> MTARIALASLFVVAAVLAQPWQTTTQRWVLGVSIAAVIVLLAWWKGMFLTTRIGRALAMVRRNRAEDTVETDAHRATVVLRVDPAAPAQLPVVVGYLDRYGITCDKVRITHRDAGGTRRSWISL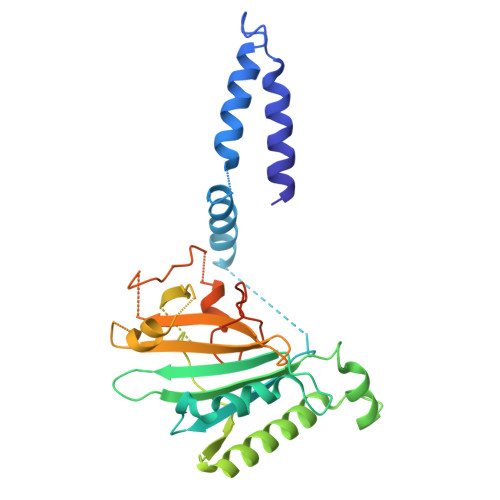TVDAVDNLAALQARSARIPLQDTTEVVGRRLADHLREQGWTVTVVEGVDTPLPVSGKETWRGVADDAGVVAAYRVKVDDRLDEVLAEIGHLPAEETWTALEFTGSPAEPLLTVCAAVRTSDRPAAKAPLAGLTPARGRHRPALAALNPLSTERLDGTAVPLPAVVRTSVKGSVEHEAAQEAGHPA> METKPRTPVLWLHGLECTCCSESFIRSAHPLAKDVVLSMISLDYDDTLMAAAGHQAEAILEEIMTKYKGNYILAVEGNPPLNQDGMSCIIGGRPFIEQLKYVAKDAKAIISWGSCASWGCVQAAKPNPTQATPVHKVITDKPIIKVPGCPPIAEVMTGVITYMLTFDRIPELDRQGRPKMFYSQRIHDKCYRRPHFDAGQFVEEWDDESARKGFCLYKMGCKGPTTYNACSTTRWNEGTSFPIQSGHGCIGCSEDGFWDKGSFYDRLTGIS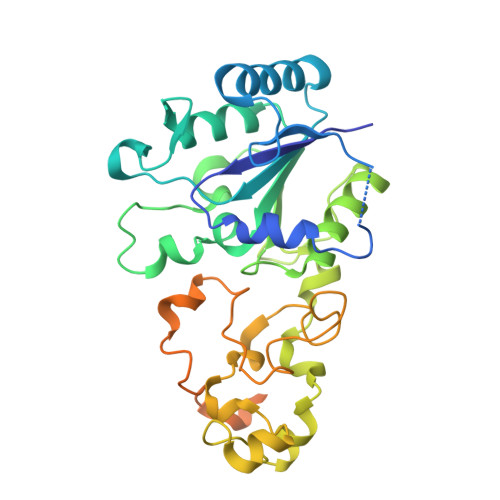QFGVEANADKIGGTASVVVGAAVTAHAAASAIKRASKKNETSGSEHRSAWSHPQFEK>[2x]MGSSHHHHHHSQDPMGQVLPLVTRQGDRIAIVSGLRTPFARQATAFHGIPAVDLGKMVVGELLARSEIPAEVIEQLVFGQVVQMPEAPNIAREIVLGTGMNVHTDAYSVSRACATSFQAVANVAESLMAGTIRAGIAGGADSSSVLPIGVSKKLARVLVDVNKARTMSQRLKLFSRLRLRDLMPVPPAVAEYSTGLRMGDTAEQMAKTYGITREQQDALAHRSHQRAAQAWSDGKLKEEVMTAFIPPYKQPLVEDNNIRGNSSLADYAKLRPAFDRKHGTVTAANSTPLTDGAAAVILMTESRAKELGLVPLGYLRSYAFTAIDVWQDMLLGPAWSTPLALERAGLTMSDLTLIDMHEAFAAQTLANIQLLGSERFAREALGRAHATGEVDDSKFNVLGGSIAYGHPFAATGARMITQTLHELRRRGGGFGLVTACAAGGLGAAMVLEAE;> MEMTSAFTLNVRLDNIAVITIDVPGEKMNTLKAEFASQVRAIIKQLRENKELRGVVFVSAKPDNFIAGADINMIGNCKTAQEAEALARQGQQLMAEIHALPIQVIAAIHGACLGGGLELALACHGRVCTDDPKTVLGLPEVQLGLLPGSGGTQRLPRLIGVSTALEMILTGKQLRAKQALKLGLVDDVVPHSILLEAAVELAKKERPSSRPLPVRERILAGPLGRALLFKMVGKKTEHKTQGNYPATERILEVVETGLAQGTSSGYDAEARAFGELAMTPQSQALRSIFFASTDVKKDPGSDAPPAPLNSVGILGGGLMGGGIAYVTACKAGIPVRIKDINPQGINHALKYSWDQLEGKVRRRHLKASERDKQLALISGTTDYRGFAHRDLII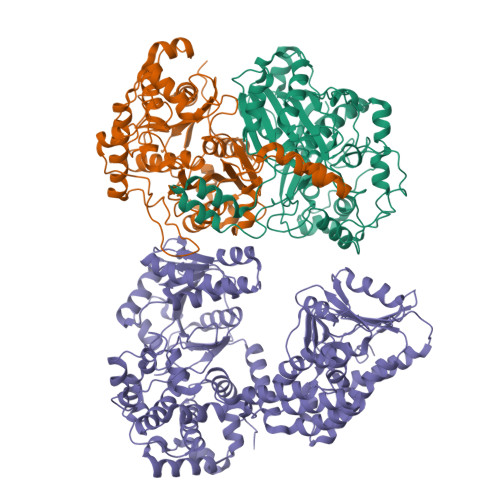EAVFENLELKQQMVAEVEQNCAAHTIFASNTSSLPIGDIAAHATRPEQVIGLHFFSPVEKMPLVEIIPHAGTSAQTIATTVKLAKKQGKTPIVVRDKAGFYVNRILAPYINEAIRMLTQGERVEHIDAALVKFGFPVGPIQLLDEVGIDTGTKIIPVLEAAYGERFSAPANVVSSILNDDRKGRKNGRGFYLYGQKGRKSKKQVDPAIYPLIGTQGQGRISAPQVAERCVMLMLNEAVRCVDEQVIRSVRDGDIGAVFGIGFPPFLGGPFRYIDSLGAGEVVAIMQRLATQYGSRFTPCERLVEMGARGESFWKTTATDLQ Although it is annotated DsbA-like, PmScsC is a powerful protein disulfide isomerase that is able to refold and reactivate the scrambled disulfide form of the model substrate RNase A just as rapidly as the archetypal disulfide isomerase E. coli DsbC. Unexpectedly, evidence from chemical cross-linking, small angle X-ray solution scattering and multi-angle light scattering all indicated that PmScsC is trimeric. The N-terminal residues bring three catalytic domains together into a trimer, and a unique flexible linker enables extraordinary twisting and extending motions that impact on the catalytic domain placement. The combination, extent and diversity of these motions would enable mis-folded substrates bound to PmScsC to explore a broad folding landscape, consistent with the redox foldase activity of this key P. mirabilis copper resistance protein.

The three crystal structures—which we refer to as compact, transitional and extended —reveal an extraordinary range of motion in this protein. Importantly, the compact and transitional structures have multiple protomers in the asymmetric unit that adopt the same overall structures in each case (8 compact trimers, RMSD ∼1.5 Å for 645 Cα; two transitional trimers, RMSD 0.5 Å for 653 Cα) so that crystal symmetry does not appear to impact on the observed conformation. Moreover, the compact and transitional conformations were determined from crystals grown under similar conditions (2.85 M sodium malonate pH 5.8, 20 °C with either 0.1 M cobalt or copper added). Nevertheless, comparison of the eight compact and the two transitional trimers in these two crystal structures, reveals an unprecedented level of conformational re-arrangement (RMSDs>20 Å). In the transitional PmScsC crystal structure, each of the two trimers incorporates protomers in three conformations: compact, extended-like and intermediate. The two compact protomer conformations of the transitional structure are similar to those in the compact crystal structure (RMSD 0.9–1.8 Å for 188 Cα). The two extended-like protomer conformations of the transitional structure are similar to the protomer in the extended crystal structure though they bend at different points in the linker helix, giving rise to somewhat different catalytic domain placements. The two intermediate conformations in the transitional crystal structure have a linker that forms a short β-strand, and positions the catalytic domain directly above the trimerization stalk. The two intermediate PmScsC crystal structures are asymmetric flat triangles with dimensions 105 × 40 × 70 Å3.

>SNAALNAAQEKEVRALVRDTLVSNPEILEEAIMALQTKKADEQQAQFRQALASEHDALYNDAASPRIGAKDAKLVLVSFTDYNCPYCKRFDPLLEKITEQYPDVAVIIKPLPFKGESSAKASQAVLSVWKEDPKAFLALHQRLMQKKTMLDNASIEDAMKSTNTSKIKLTDDSLKTLQNNLELSRKLGIQGTPATVIGDTILPGAVDYDQLEIIVKEQLAKVKK[6x]>GSSHHHHHHSSGLVPRGSPQPPADEQPEPRTRRRAYLWCKEFLPGAWRGLREDEFHISVIRGGLSNMLFQCSLPDTTATLGDEPRKVLLRLYGAILQMRSCNKEGSEQAQKENEFQGAEAMVLESVMFAILAERSLGPKLYGIFPQGRLEQFIPSRRLDTEELSLPDISAEIAEKMATFHGMKMPFNKEPKWLFGTMEKYLKEVLRIKFTEESRIKKLHKLLSYNLPLELENLRSLLESTPSPVVFCHNDCQEGNILLLEGRENSEKQKLMLIDFEYSSYNYRGFDIGNHFC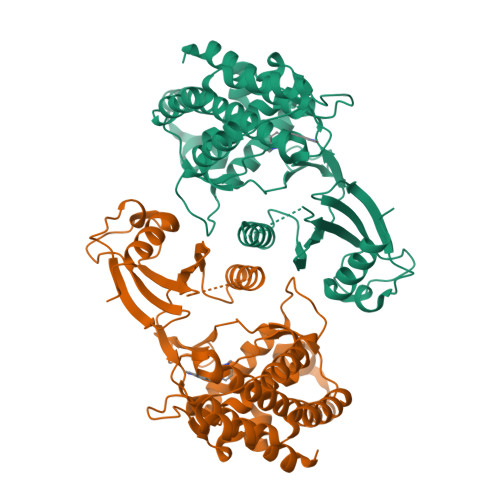EWMYDYSYEKYPFFRANIRKYPTKKQQLHFISSYLPAFQNDFENLSTEEKSIIKEEMLLEVNRFALASHFLWGLWSIVQAKISSIEFGYMDYAQARFDAYFHQKRKLGV[2x]> MENKIEVNSKDEMNKWFEEFKKGNGLVDTYTNSYSFCESVPNLDRFVFQMAGATDDAQKDSIYASALVEATKFCAPIYECAWASSTGIVKKGLEWFEKNTGTIKSWDESYIELKVEVPKIEQLFNYQQAALKWRKDIGFRVNANTAALSNKVLAEYKVPGEIVMSVKEMLSDMIRRRNLILNRGGDENPRGPVSHEHVEWCREFVKGKYIMAFNPPWGDINKSGRSGIALVATGLAKLAETEGKGVFDEAKKT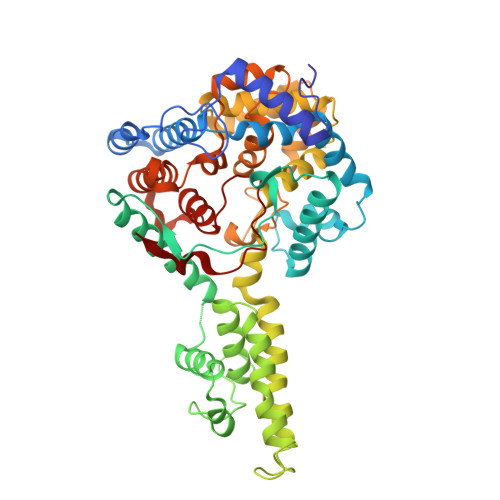VEALNGYLDKHKDEVDKASADNMVTNLLKHVAKAQELYKNSSALRAQGAQIDTVFSSYYWLYKAGVTPETFPTVSQFLFELGKHPRGTKKMKKALLSTPMKWGKKLYELFADDSFQQNRIYMHPAVLTAGRISEMGVCFGTIPVANPDDAALGSGHTKSILNLRTNTETNNPCARTIVKLFEIQKTGFNIQDMDIVASEHLLHQSLVGKQSPFQNAYNVKGNATSANII>MNHKVHHHHHHIEG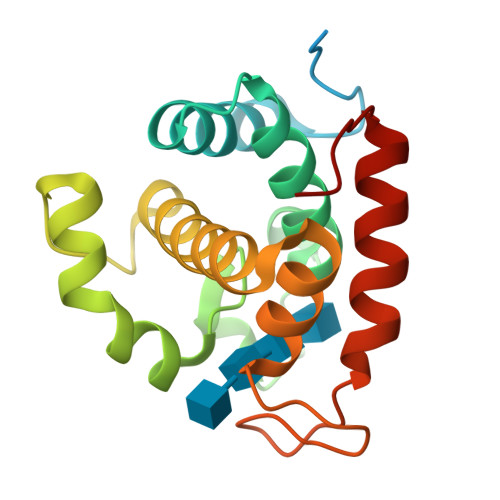RHMGTTPSDPPTNPPTTVTKPAEVPSRIWTYVMNADNAYGKGGDFALLLSAVIKKQSYFGDGLSGSPSAGDGLMQVEPNTRNAYLSQFSAKYGHAYNHSSEQDQVYMGSLILNEKIVRFGSIYSGLLHYNGGDYWYPGATDSYGRPILADQYANTVYAQYKSYGGRYSR[4x]>[2x]GSSSTLTKELIKDAAEKCCTRNRQECCIEIMKFGTPIRCGYDRDPKLPGYVYKCLQNVLFAKEPKKKINLDDSVCCSVFGNDQEDSGRRCENRCKNLMTSPSIDAATRL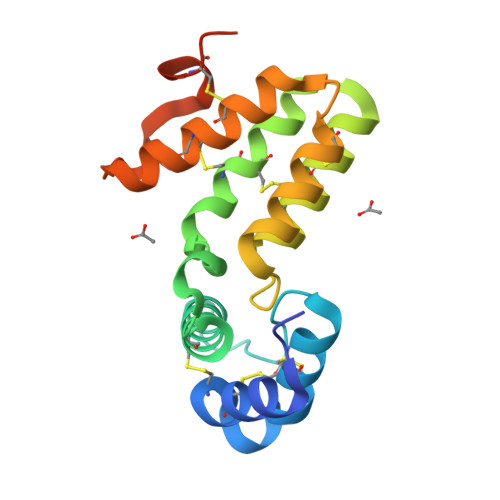DSIKSCSLLDNVLYKCFEKCRSLRKDGIKIEVLQFEEYCEATFIQKRTFRGV>[2x]MAKDATQGGVQALSAWTNQSGSTLYIQSVDPSGSLSGYYINRAAGYGCQNTPYPVTGWVYGTAITFTVLWENATESCNSITA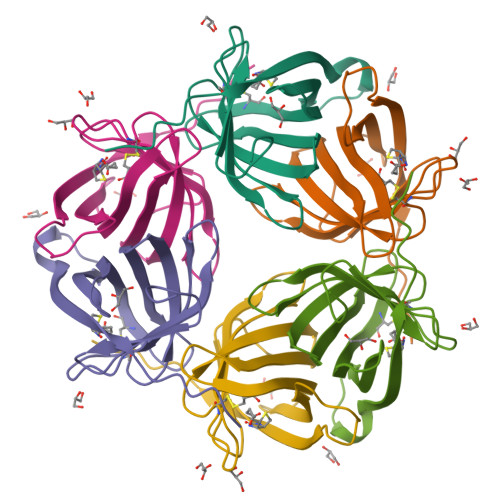WTGFYYQGQITTLWQLVINGSTSTGQIISGEDIFKPSQQKKSKTLKGK> YFQSMPVKTGSPTFVRELRSRTFDSSDEVILKPTGNQLTVEFLEENSFSVPILVLKKDGLGMTLPSPSFTVRDVEHYVGSDKE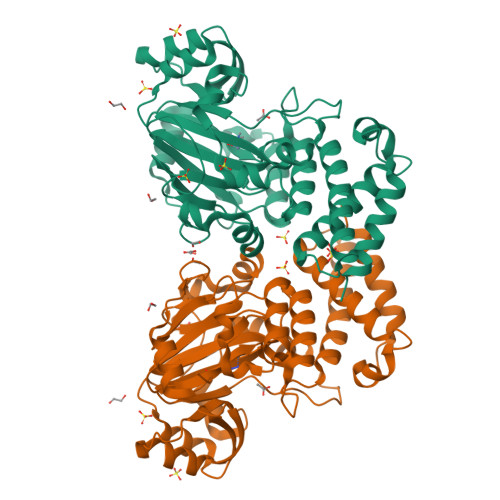IDVIDVTRQADCKMKLGDFVKYYYSGKREKVLNVISLEFSDTRLSNLVETPKIVRKLSWVENLWPEECVFERPNVQKYCLMSVRDSYTDFHIDFGGTSVWYHVLKGEKIFYLIRPTNANLTLFECWSSSSNQNEMFFGDQVDKCYKCSVKQGQTLFIPTGWIHAVLTPVDCLAFGGNFLHSLNIEMQLKAYEIEKRLSTADLFRFPNFETICWYVGKHILDIFRGLRENRRHPASYLVHGGKALNLAFRAWTRKEALPDHEDEIPETVRTVQLIKDLAREIRLVEDIFQQN>[2x]FTPVTKAAVINTFDG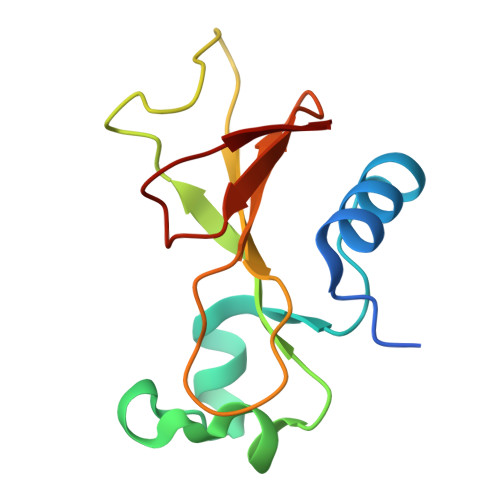VADYLIRYKRLPNDYITKSQASALGWVASKGDLAEVAPGKSIGGDVFSNREGRLPSAGSRTWREADINYVSGFRNADRLVYSSDWLIYKTTDHYATFTRIR>[4x]MNYQNDDVRVKQIKELLPPIALLEKFPATDKAAFTVHEARHAIHNILVGKDDRLVVVIGPCSIHDTKAALEYAERLKEIREELKDSLEIVMRVYFEKPRTTVGWKGLINDPHMDHSFDINEGLRIARELLLTINDQGLPTAGEFLDVISPQYVADLMSWGAIGARTTESQIHRELASGLSCPVGFKNGT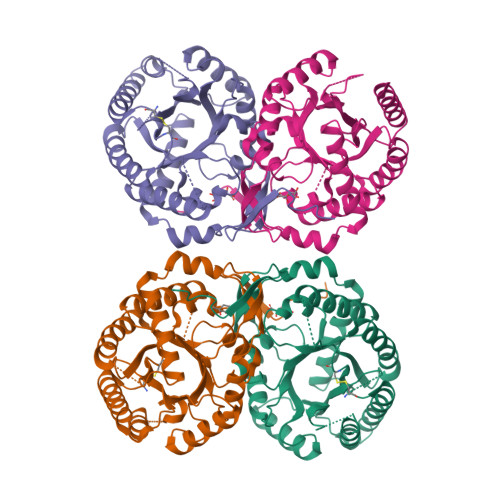DGTIKIAIDAINSARSAHSFLSVTKWGHSAIVNTSGNPDCHIILRGGKEPNYSAEHVKAVREGLINAGLIPSIMIDFSHANSSKKFEKQMEVATDVSTQLSQGDRSITGVMIESHLVEGNQNLESGEPLVYGKSVTDACIGWDDTEKVLRQLSEAVIARRNK TMEM16A, a calcium-activated chloride channel involved in multiple cellular processes, is a proposed target for diseases such as hypertension, asthma, and cystic fibrosis. The protein is broadly expressed and mediates vital physiological functions including fluid secretion, smooth muscle contraction, and the control of electrical signaling in certain neurons. TMEM16A is a homodimer with each subunit containing an ion conduction pore. Both pores act independently and are activated by the binding of two Ca2+ ions from the cytoplasm to a conserved site situated in the proximity of the ion conduction path.

With an overall resolution of 2.85 Å, the final map shows well-defined density for the entire protein, including two Ca2+ ions bound at the canonical transmembrane site and at an additional site near the dimer interface that was originally identified in the structures of TMEM16K30 and F31 and whose involvement in channel activation has recently been demonstrated in TMEM16A29. Non-protein density, which is not present in any of the previous maps of TMEM16A, is found at the extracellular end of the hourglass-shaped pore of each subunit. The location of the site within the transmembrane electric field, with a fractional voltage drop of ~0.2 as estimated from Poisson-Boltzmann calculations, is consistent with the voltage dependence and the perceived mechanism of block obtained from functional experiments. The binding site is complementary to the blocker in both its shape and polarity. The binding of the blocker stabilizes an open-like conformation of the channel that involves a rearrangement of several pore helices. A much more extended transition is found in α3, where the rearrangement of the helix changes its tilt and results in a clockwise rotation of about 60° around its axis and an upward shift of about 6 Å from the Ca2+-free to the Ca2+-bound state. The outward movement of α4 widens the outer pore entrance, while the more extended conformational change of α3 relocates Tyr 514 away from the pore and projects the adjacent Arg 515 towards the pore lumen, creating a site that accommodates the blocker. The binding of the blocker to the site immediately external to the narrow neck results in a direct blockade of the ion conduction path, thereby inhibiting channel activity. Collectively, the described conformational changes result in major rearrangements of residues on α3, including the positively charged Arg 515 and the hydrophobic Val 508, Val 511, and Ile 512 that are all in contact with the bound blocker, and a comparatively smaller repositioning of pore-lining residues on α4 and 6, including Val 543, Asn 546, and Ile 551 that have partially retracted from the pore lumen.

>[2x]MRVPEKYSTLPAEDRSVHIVNICAIEDLGYLPSEGTLLNSLSVDPDAECKYGLYFRDGKRKVDYILVYHHKRASGSRTLARRGLQNDMVLGTRSVRQDQPLPGKGSPVDAGSPEVPMDYHEDDKRFRREEYEGNLLEAGLELENDEDTKIHGVGFVKIHAPWHVLCREAEFLKLKMPTKKVYHISETRGLLKTINSVLQKITDPIQPKVAEHRPQTTKRLSYPFSREKQHLFDLTDRDSFFDSKTRSTIVYEILKRTTCTKAKYSMGITSLLANGVYSAAYPLHDGDYEGDNVEFNDRKLLYEEWASYGVFYKYQPIDLVRKYFGEKVGLYFAWLGAYTQMLIPASIVGVIVFLYGCATVDENIPSMEMCDQRYNITMCPLCDKTCSYWKMSSACATARASHLFDNPATVFFSVFMALWAATFMEHWKRKQMRLNYRWDLTGFEEEEEAVKDHPRAEYEARVLEKSLRKESRNKETDKVKLTWRDRFPAYFTNLVSIIFMIAVTFAIVLGVIIYRISTAAALAMNSSPSVRSNIRVTVTATAVIINLVVIILLDEVYGCIARWLTKIEVPKTEKSFEERLTFKAFLLKFVNSYTPIFYVAFFKGRFVGRPGDYVYIFRSFRMEECAPGGCLMELCIQLSIIMLGKQLIQNNLFEIGIPKMKKFIRYLKLRRQSPSDREEYVKRKQRYEVDFNLEPFAGLTPEYMEMIIQFGFVTLFVASFPLAPLFALLNNIIEIRLDAKKFVTELRRPVAIRAKDIGIWYNILRGVGKLAVIINAFVISFTSDFIPRLVYLYMYSQNGTMHGFVNHTLSSFNVSDFQNGTAPNDPLDLGYEVQICRYKDYREPPWSEHKYDISKDFWAVLAARLAFVIVFQNLVMFMSDFVDWVIPDIPKDISQQIHKEKVLMVELFMREEQGKQQLLDTWMEKEKPRDVPCNNHSPTTHPEAGDGSPVPSYEYHGDAL> UGGAAGAAAUCGAAGAAGAUGAAGAACGCGAAGAAC;> AUCUUCUUCGAUUUCUUCCAGUUCUUCGCGUUCUUC

Recently, RNA-catalyzed rolling circle synthesis (RCS) on small circular RNA (scRNA) templates has been demonstrated. To gain deeper insight into the RCS process and the strong inhibition observed upon full-length circle synthesis, we used cryo-EM to study the structure of putative RCS replication products formed by complexing the full-length scRNA and nascent complementary RNA (cmpRNA). To our surprise, cryo-EM revealed not one by a diverse variety of distinct structural species identified as monomers, dimers, and multimers of the scRNA–cmpRNA complex. We find that scRNAs and cmpRNAs of 36 nt in length can form an unanticipated diversity of structures with different stoichiometries, including a fully annealed dimer (comprising two scRNAs and two cmpRNAs) and multimers hereof.

Class 1 showed a density corresponding to two helical turns of an RNA double helix. The low-resolution cryo-EM maps of classes 1 and 2 are consistent with partly hybridized scRNA and cmpRNA. The density map for class 1 was observed to have slightly more than two helical turns. The density was analyzed by aligning a model of the scRNA–cmpRNA complex that was previously predicted by MD simulation to form ∼24 bp. The similarity between the class 1 map and the MD model suggests that they could represent the same species. Based on this hypothesis, we constructed a new 3D model of the whole system that fits the class 1 density. Note that the cryo-EM density shows only the double-stranded segment, making the placement of the single-stranded regions ambiguous. The single-stranded regions are not seen in the map because they are flexible and are averaged out during 3D reconstruction. In class 1, only ∼66% of the possible base pairs are formed (∼24 bp out of 36 bp); in class 2, ∼80% are formed (∼58 bp out of 72 bp); and in class 3, 100% are formed (72 bp out of 72 bp). The folding path begins with the annealing of scRNA and cmpRNA to form class 1 monomers with a 24-bp annealing region.(2~{R},3~{R},4~{S},5~{S})-2-[2,6-bis(azanyl)purin-9-yl]-5-(methylsulfanylmethyl)oxolane-3,4-diol | C11 H16 N6 O3 S | 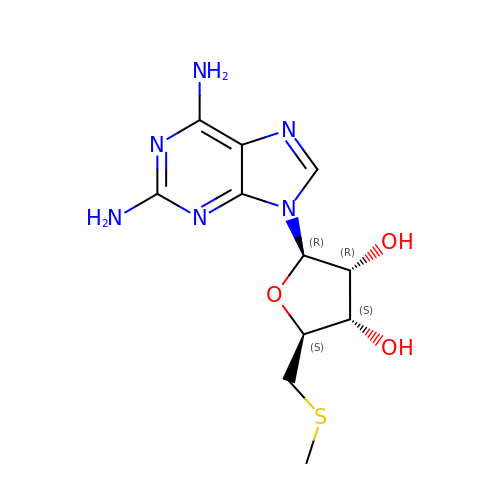POSHIZZVLUQFIQ-KQYNXXCUSA-N> MTKPLDGINVLDFTHVQAGPACTQMMGFLGANVIKIERRGSGDMTRGWLQDKPNVDSLYFTMFNCNKRSIELDMKTPEGKELLEQMIKKADVMVENFGPGALDRMGFTWEYIQELNPRVILASVKGYAEGHANEHLKVYENVAQCSGGAAATTGFWDGPPTVSGAALGXSNSGMHLMIGILAALEIRHKTGRGQKVAVAMQDAVLNLVRIKLRDQQRLERTGILAEYPQAQPNFAFDRDGNPLSFDNITSVPRGGNAGGGGQPGWMLKCKGWETDADSYVYFTIAANMWPQICDMIDKPEWKDDPAYNTFEGRVDKLMDIFSFIETKFADKD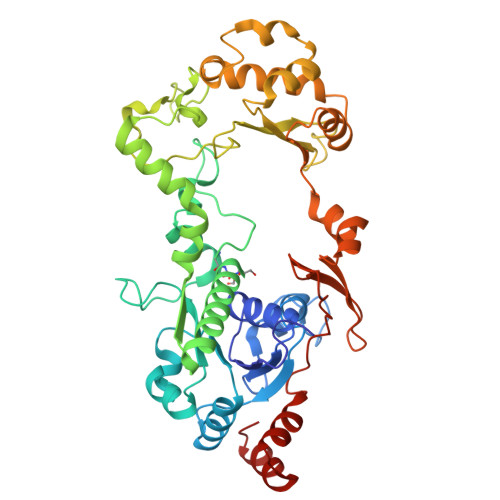KFEVTEWAAQYGIPCGPVMSMKELAHDPSLQKVGTVVEVVDEIRGNHLTVGAPFKFSGFQPEITRAPLLGEHTDEVLKELGLDDAKIKELHAKQVV> GSHMTRETERFPAREFQRDLLDWFARERRDLPWRKDRDPYKVWVSEVMLQQTRVETVIPYFEQFIDRFPTLEALADADEDEVLKAWEGLGYYSRVRNLHAAVKEVKTRYGGKVPDDPDEFSRLKGVGPYTVGAVLSLAYGVPEPAVNGNVMRVLSRLFLVTDDIAKCSTRKRFEQIVR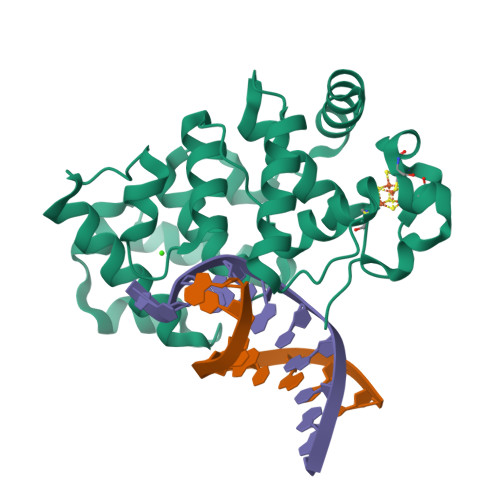EIMAYENPGAFNEALIELGALVCTPRRPSCLLCPVQAYCQAFAEGVAEELPVKM> SIVSKSIVNADAEARYLSPGELERIKTFVVGGDRRLRIA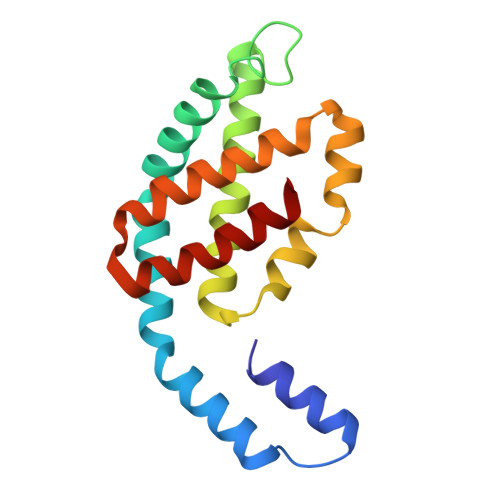QTIAESRERIVKQAGNQLFQKRPDVVSPGGNAYGEDMTATCLRDLDYYLRLVTYGVVSGDITPIEEIGIVGVREMYKSLGTPIEAVAEGVRELKSAATALLTGEDADEAGAYFDYVIGALS>SSQLHVAIVSSPGMGHLIPVLVLGNRLATHHNIKITILAITTTSSSAETEFLKKTTLTNEEKTIEIIPVPSVDISHLINSSTKIFTQLRLLVREALPKIHSTIASMTHRPDALIVDIFCTQILPIAEEFNISKYTYHPTTAWTLALAIYCQVFDKEIEGEYVELKEPLKIPGCKALRPDDVVDPLLDRSDQQYEEYVKLGKEYTDFDGILINTWEDLEPETINALRYNEKLRLLLKVPVFPIGPLRRKVETTLNDEVIQWLDKQNNESVLFVSFGSGGTLSTKQMTELAWGLELSQQKFVWVVRPPSDGDADSAYLNSAGKDTRDMSEYLPEGFLTRTKDMGLVVPMWANQVEILSHSSVGGFLTHCGWNSTVESLTNGVPMIAWPLHAEQK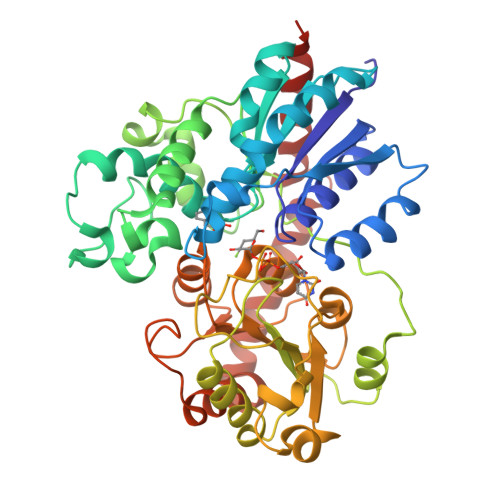MNAAMLTEELGVAIRPAVLPTKKLVKREEIQGMVRILMQTKEGKRIKEKAKKLKKSAENALSDGGSSYNSICELVKDIRSREL[2x]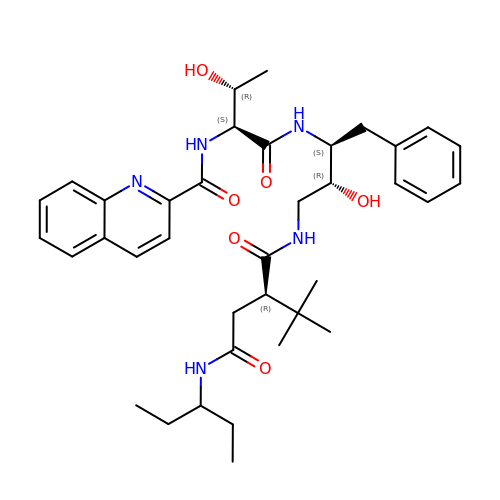(2S)-2-tert-butyl-N~4~-(1-ethylpropyl)-N~1~-[(2R,3S)-2-hydroxy-4-phenyl-3-{[N-(quinolin-2-ylcarbonyl)-L-threonyl]amino}butyl]butanediamide | C37 H51 N5 O6 | LUQGXGNLGWQNMB-BJPNTFJISA-N>[3x]MMFGRFTERAQKVLALAQEEALRLGHNNIGTEHILLGLVREGEGIAAKALQALGLGSEKIQKEVESLIGRGQEMSQTIHYTPRAKKVIELSMDEARKLGHSYVGTEHILLGLIREGEGVAARVLNNLGVSLNKARQQVLQLLGSNETGSSAAGTNSNANTPTLDSLARDLTAIAKEDSLDPVIGRSKEIQRVIEVLSRRTKNNPVLIGEPGVGKTAIAEGLAQQIINNEVPEILRDKRVMTLDMGTKYRGEFEDRLKKVMDEIRQAGNIILFIDAAIDASNILKPSLARGELQCIGATTLDEYRKYIEKDAALERRFQPIQVDQPSVDESIQILQGLRDRYEAHHRVSITDDAIEAAVKLSDRYISDRFLPDKAIDLIDEAGSKVRLRSFTTPPNLKELEQKLDEVRKEKDAAVQSQEFEKAASLRDTEQRLREQVEDTKKSWKEKQGQENSEVTVDDIAM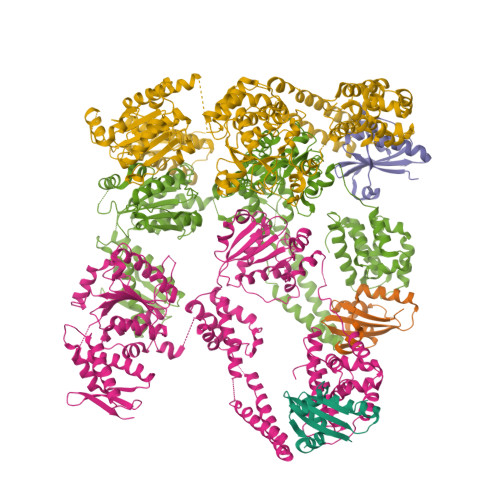VVSSWTGVPVSKIAQTETDKLLNMENILHSRVIGQDEAVVAVAKAVRRARAGLKDPKRPIGSFIFLGPTGVGKTELARALAESIFGDEESMIRIDMSEYMEKHSTSGGQLTEKVRRKPYSVVLLDAIEKAHPDVFNILLQVLEDGRLTDSKGRTVDFRNTILIMTSNVGASEKDKVMGELKRAFRPEFINRIDEIIVFHSLEKKHLTEIVSLMSDQLTKRLKEQDLSIELTDAAKAKVAEEGVDLEYGARPLRRAIQKHVEDRLSEELLRGNIHKGQHIVLDVEDGEFVVKTTAKTN;>[3x]LDDFQKEEQAVNQEEKEQKLQFVLRFGDFEDVISLSKLNVNGSKTTLYSFENRYYLYVDFCNMTDEEVENQLSILLEYATESSISIHRLEEYGKLIISEHALETIKKHFAS Here, we demonstrate the determination of the crystal structures of T. brucei GMPR; a protein that, unlike the GMPRs of host animals, possesses a CBS domain. We further show that TbGMPR activity is regulated by purine nucleotide binding to an allosteric regulatory site formed at the cleft between the catalytic and CBS domains of the enzyme. Our kinetic and structural analyses clearly demonstrate that the CBS domain has a pivotal role in the allosteric regulation of the activity and structure of TbGMPR, facilitating the transitions among three conformations: a tetramer, and octamers with relaxed and twisted conformations. A combination of X-ray crystallography and size-exclusion chromatography small-angle X-ray scattering (SEC-SAXS) analysis clearly revealed that TbGMPR can exist as a tetramer or an octamer depending on the nucleotide species that is bound to the CBS domain.

We further determined the structure of the wild-type TbGMPR complexed with GTP (TbGMPR/GTP) at 2.50-Å resolution. In this structure, single GTP molecules were found only at the allosteric regulatory site on each subunit of TbGMPR/GTP, indicating that GTP acts only as a ligand. The overall structure was almost identical to that of C318A/GMP (RMSD = 0.66 Å for Cα atoms). The hinge motion in each subunit and the twisted conformation of the octamer upon allosteric binding of the ligand were also observed in TbGMPR/GTP. The present crystallographic study of TbGMPR shows that both GMP and GTP share the canonical site 2 on the CBS domain, whereas nothing was observed on the canonical site 1. However, the affinity of GTP to the canonical site 2 was higher than that of GMP as observed in the fluorescence quenching assay. These findings indicate that, in the presence of sufficient concentration of GTP, GMP no longer activates TbGMPR since the canonical site 2 has been occupied by GTP. Consequently, the kinetics of TbGMPR in the presence of GTP shows a Michaelis–Menten-like profile with a decrease of the nHill value to ~1. In the presence of GTP, the initial velocity of TbGMPR was upregulated in a concentration-dependent manner, and the EC50 value was estimated to be 4.8 µM. The addition of GTP to the reaction mixture enhanced TbGMPR activity by decreasing the K0.5 accompanied with the increase of the kcat value in a concentration-dependent manner.

> MSFNESASIPTGLTYDDVLIIPQHSRVTSRKEVNTTTRLSRNVKLSIPIVASNMDTVCEQRMAVAMAREGGIGILHRFCSIEEQCAMLREVKRAQSFLIESPRIILPHETAREAWEGLNWKGRVGGVGCLLVVNCKNERKLLGIITRHDLKLADESTTVESLMTPVDKMVVSTNTSISLEEVTHLMRKGRTANVPIVGQNGQLLYLVTLSDVVKLRKNKQASLDSRGRLLVGAAVGVKKDDMNRAIRLVEAGADVLVVDIAHGHSDLCINMVKRLKGDPRTASVDIIAGNIASAEAAEALIDAGADGLKIGVGPGSICITRLVAGAGVPQLSAVLACTRVARRRGVPCIADGGLRTSGDISKAIGAGADTVMLGNMLAGTDEAPGRVLVKDGQKVKIIRGMAGFGANLSKAERERTQDEDVFSSLVPEGVEGSVACKGPVGPIVRQLVGGLRSGMSYSGAKSIEEMQRRTRFVRMTGAGLRESGSHGVAKLKLAAALEHHHHHH>[4x]MGNLTGNSKKAADSGDKPVIKMYQIGDKPDNLDELLANANKIIEEKVGAKLDIQYLGWGDYGKKMSVITSSGENYDIAFADNYIVNAQKGAYADLTELYKKEGKDLYKALDPAYIKGNTVNGKIYAVPVAANVASSQNFAFNGTLLAKYGIDISGVTSYETLEPVLKQIKEKAPDVVPFAIGKVFIP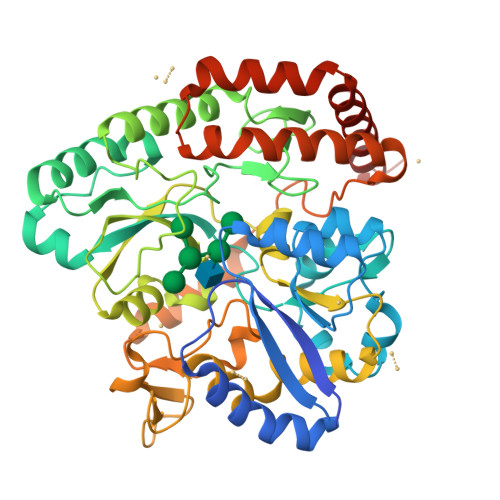SDNFDYPVANGLPFVIDLEGDTTKVVNRYEVPRFKEHLKTLHKFYEAGYIPKDVATSDTSFDLQQDTWFVREETVGPADYGNSLLSRVANKDIQIKPITNFIKKNQTTQVANFVISNNSKNKEKSMEILNLLNTNPELLNGLVYGPEGKNWEKIEGKENRVRVLDGYKGNTHMGGWNTGNNWILYINENVTDQQIENSKKELAEAKESPALGFIFNTDNVKSEISAIANTMQQFDTAINTGTVDPDKAIPELMEKLKSEGAYEKVLNEMQKQYDEFLKNKKLEHHHHHH>GSLVLSELSQGLAVELMERVMMEFVRETCSQELKNAVETDQRVRVARCCEDVCAHLVDLFLVEEIFQTAKETLQE[2x];>[4x]MVVSKMNKDAQMRAAINQKLIETGERERLKELLRAKLIECGWK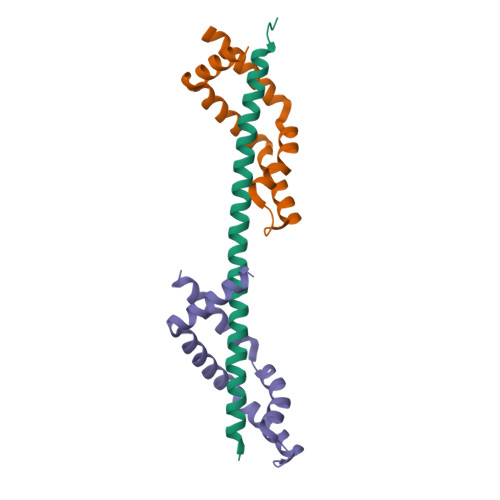DQLKAHCKEVIKEKGLEHVTVDDLVAEITPKGRALVPDSVKKELLQRIRTFLAQHASL> MAHHHHHHNPNYCFAGKTSSISDLKEVPRKNITLIRGLGHGAFGEVYEGQVSGMPNDPSPLQVAVKTLPEVCSE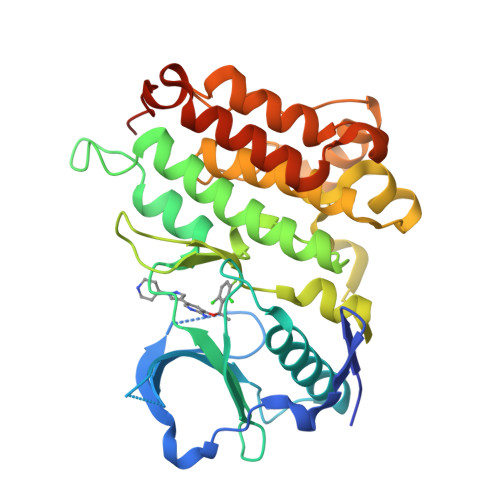QDELDFLMEALIISKFNHQNIVRCIGVSLQSLPRFILMELMAGGDLKSFLRETRPRPSQPSSLAMLDLLHVARDIACGCQYLEENHFIHRDIAARNCLLTCPGPGRVAKIGDFGMARDIYRASYYRKGGCAMLPVKWMPPEAFMEGIFTSKTDTWSFGVLLWEIFSLGYMPYPSKSNQEVLEFVTSGGRMDPPKNCPGPVYRIMTQCWQHQPEDRPNFAIILERIEYCTQDPDVINTALPIEYGPLVEEEEKV> MMSFQKIYSPTQLANAMKLVRQQNGWTQSELAKKIGIK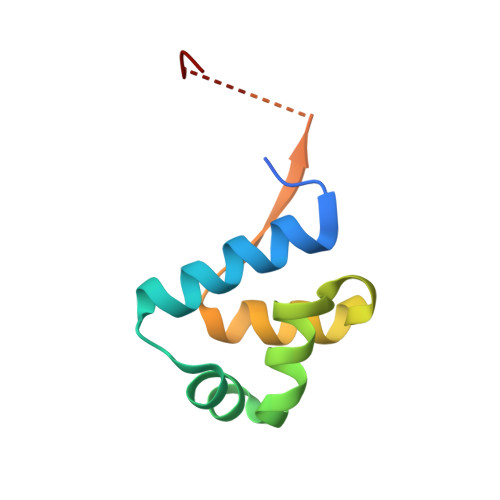QATISNFENNPDNTTLTTFFKILQSLELSMTLCDAKNASPESTEQQNLEW> KRYIPSVNDFVIGVIIGTFSDSYKVSLQNFSSSVSLSYMAFPNASKKNRPTLQVGDLVYARVCTAEKELEAEIECFDSTTGRDAGFGILEDGMIIDVNLNFARQLLFNNDFPLLKVLAAHTKFEVAIGLNGKIWVKCEELSNTLACYRTIMECCQKNDTAAFKD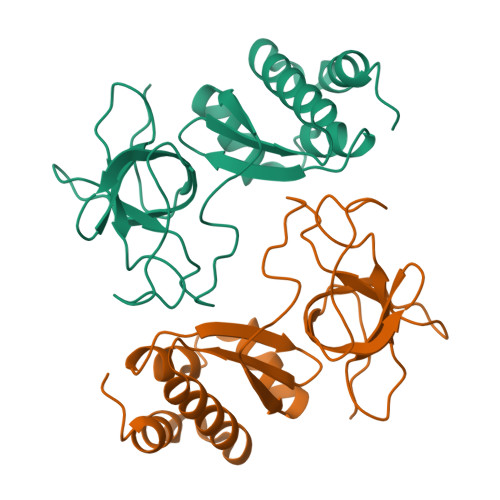IAKRQFKEILT> ADSLSIPPVKAGAKQLPMPSVSGAQIKLLGADYEQLVNSKGKIAPVISDTP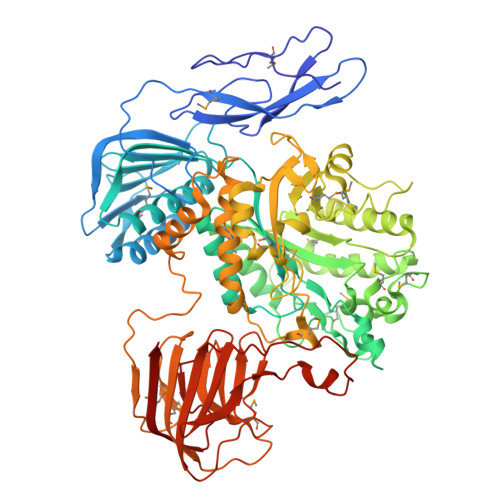VNVSFKVTKDGKEAVSKDYEIMLQAPQAAQGNPKPRIIPEILQWKGGQGEYKLGNTVTIACPDKELGKLFAADMEDVLGKKVKLVAPGAKADISLSLLKGGNLGREGYRLQIARDGVRLGAAAPTGLFWGTRTLLQMLRQTPGSVPCGTAVDFPRYQLRGFMLDVARTPYPLSYLKDVIRTMAWYKMNDLHLVINNNYIFHEHYVDNGHDPFKESYAAFRLESKMKGKDGTPLTARDLFYTKKEFADLVSYARKYGVNIVPEFDTPGHALSFTRLRPDLIYKGPMNHEKRRCEMLDAANPETIDLVSKVFDEYMLKDPKLGRPVFADCGVVHVGADEFYGDKEDYRHFANAVLTHALKRGYTPRIWGSLSAKPGKTPVVSKGVQMNLWSTGWMKAWEAVNQGYDVINTNDGALYIVPFAGYYRMDRNHKGLYNNWIPNRIGNETLPSGHPQLLGGTFAVWNDETDIMHTGYAPYDIWGIISGSMDVLSQKLWGTAKAPDTFEQHRELVSSIGNAPRTNPLHKWKDSQPLTVKPSSLPQKLDKPALGPNYRLTMELELTAAPEGKEQVLLAAPEGELLAVMKDGTVGFRRDDSLEFSFGAKLPVGKKVKVEIVGEPEKTSLLLDGEPAGTAVLKNFSDKSKDFSDKFKHRPKVHRSTFILPLKELGSSFQGKVFHMNVQPL>[4x]MAHHHHHHEPGDLRHDLNQQERATLSSNVQRFFMIGHG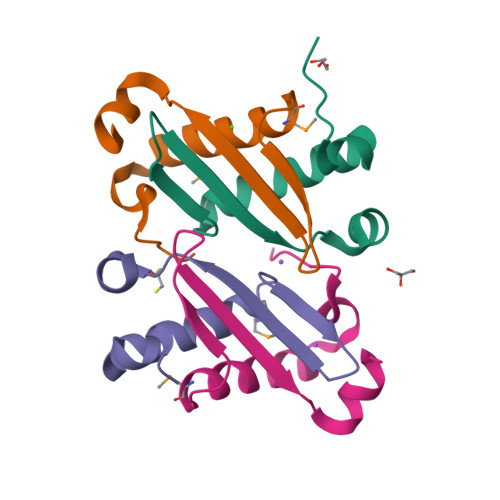SLTADAGGLTYTVSWVPTKQIQRKVAPSAGP>[2x]MTVKMGFIGFGKSANRYHLPYVMIRETLEVKTIFDLHVNEKAAAPFKEKGVNFTADLNELLTDPEIELITICTPAHTHYDLAKQAILAGKSVIVEKPFCDTLEHAEELFALGQEKGVVVMPYQNRRFDGD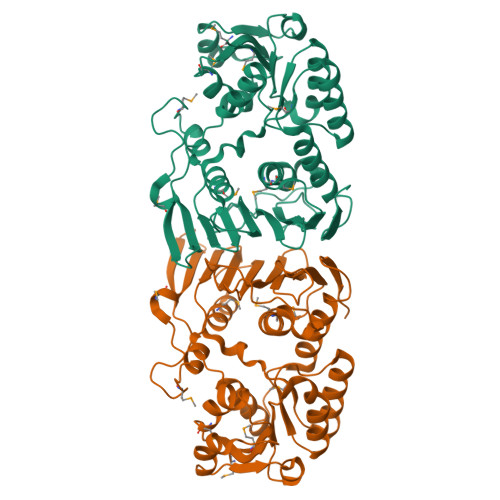YLAMKQVVEQGFLGEINEVETHIDYYRPGSITEQGPKENGSFYGLGIHLMDRMIALFGRPDQVTYDIRNNEVSEAVDNYFDVDLHYGSKLKVKVKTNHSVASPYPRFIVHGSNGSFIKYGEDQQENDLKAGIMPDAPGFGEDSPMYYGEVTYRNGNGDWIKKQIKTPVGDYGRYYDAVYETLKNGAPQLVTKEQALTNIEILEAGFLNPSPSVYHLKEN> MTDHVREADDANIDDLLGDLGGTARAERAKLVEWLLEQGITPDEIRATNPPLLLATRHLVGDDGTYVSAREISENYGVDLELLQRVQRAVGLARVDDPDAVVHMRADGEAAARAQRFVELGL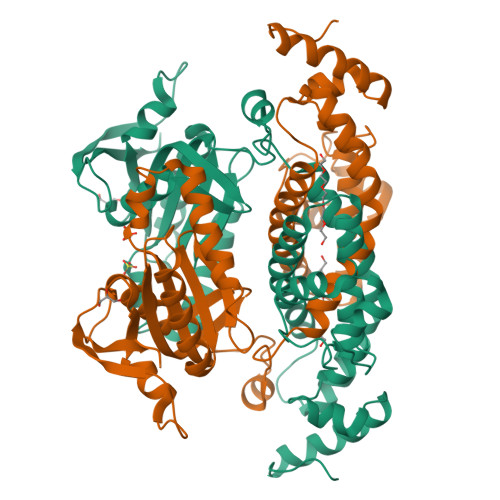NPDQVVLVVRVLAEGLSHAAEAMRYTALEAIMRPGATELDIAKGSQALVSQIVPLLGPMIQDMLFMQLRHMMETEAVNAGERAAGKPLPGARQVTVAFADLVGFTQLGEVVSAEELGHLAGRLAGLARDLTAPPVWFIKTIGDAVMLVCPDPAPLLDTVLKLVEVVDTDNNFPRLRAGVASGMAVSRAGDWFGSPVNVASRVTGVARPGAVLVADSVREALGDAPEADGFQWSFAGPRRLRGIRGDVRLFRVRRGATRTGSGGAAQDDDLAGSSPGSRSHHHHHH>MGTTTMGVMLDDATRERIKSAATRIDRTPHWLIKQAI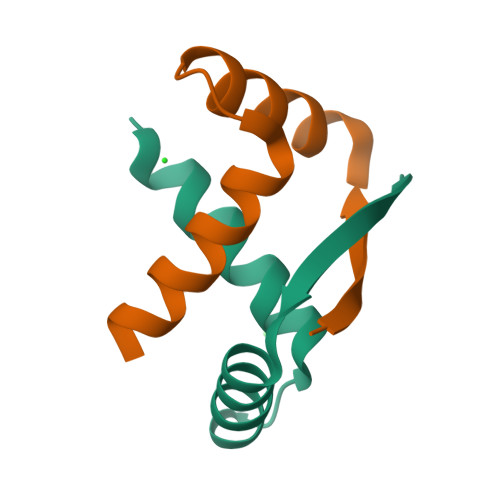FSYLEQLENSDTLPEHHHHHH[6x]> MSRESNDTIQSDTVRSSSKSDYFRIQLNNQDYYMSKPTFLDPSHGESLPLNQFSQVPNIRVFGALPTGHQVLCHVHGILPYMFIKYDGQITDTSTLRHQRCAQVHKTLEVKIRASFKRKKDDKHDLAGDKLGNLNFVADVSVVKGIPFYGYHVGWNLFYKISLLNPSCLSRISELIRDGKIFGKKFEIYESHIPYLLQWTADFNLFGCSWINVDRCYFRSPVLNSILDIDKLTINDDLQLLLDRFCDFKCNVLSRRDFPRVGNGLIEIDILPQFIKNREKLQHRDIHHDFLEKLGDISDIPVKPYVSSARDMINELTMQREELSLKEYKEPPETKRHVSGHQWQSSGEFEAFYKKAQHKTSTFDGQIPNFENFIDKNQKFSAINTPYEALPQLWPRLPQIEINNNSMQDKKNDDQVNASFTEYEICGVDNENEGVKGSNIKSRSYSWLPESIASPKDSTILLDH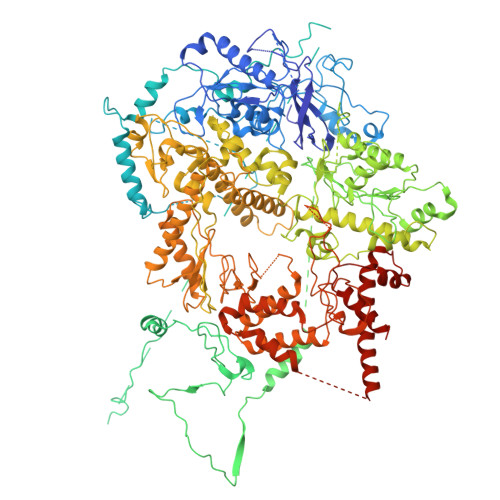QTKYHNTINFSMDCAMTQNMASKRKLRSSVSANKTSLLSRKRKKVMAAGLRYGKRAFVYGEPPFGYQDILNKLEDEGFPKIDYKDPFFSNPVDLENKPYAYAGKRFEISSTHVSTRIPVQFGGETVSVYNKPTFDMFSSWKYALKPPTYDAVQKWYNKVPSMGNKKTESQISMHTPHSKFLYKFASDVSGKQKRKKSSVHDSLTHLTLEIHANTRSDKIPDPAIDEVSMIIWCLEEETFPLDLDIAYEGIMIVHKASEDSTFPTKIQHCINEIPVMFYESEFEMFEALTDLVLLLDPDILSGFEIHNFSWGYIIERCQKIHQFDIVRELARVKCQIKTKLSDTWGYAHSSGIMITGRHMINIWRALRSDVNLTQYTIESAAFNILHKRLPHFSFESLTNMWNAKKSTTELKTVLNYWLSRAQINIQLLRKQDYIARNIEQARLIGIDFHSVYYRGSQFKVESFLIRICKSESFILLSPGKKDVRKQKALECVPLVMEPESAFYKSPLIVLDFQSLYPSIMIGYNYCYSTMIGRVREINLTENNLGVSKFSLPRNILALLKNDVTIAPNGVVYAKTSVRKSTLSKMLTDILDVRVMIKKTMNEIGDDNTTLKRLLNNKQLALKLLANVTYGYTSASFSGRMPCSDLADSIVQTGRETLEKAIDIIEKDETWNAKVVYGDTDSLFVYLPGKTAIEAFSIGHAMAERVTQNNPKPIFLKFEKVYHPSILISKKRYVGFSYESPSQTLPIFDAKGIETVRRDGIPAQQKIIEKCIRLLFQTKDLSKIKKYLQNEFFKIQIGKVSAQDFCFAKEVKLGAYKSEKTAPAGAVVVKRRINEDHRAEPQYKERIPYLVVKGKQGQLLRERCVSPEEFLEGENLELDSEYYINKILIPPLDRLFNLIGINVGNWAQEIVKSKRASTTTTKVENITRVGTSATCCNCGEELTKICSLQLCDDCLEKRSTTTLSFLIKKLKRQKEYQTLKTVCRTCSYRYTSDAGIENDHIASKCNSYDCPVFYSRVKAERYLRDNQSVQREEALISLNDW> MKSNDMNITVELTFFEPYRLVEWFDWDARKKSHSAMRGQAFAQWTWKGKGRTAGKSFITGTLVRSAVIKAVEELLSLNNGKWEGVPCCNGSFQTDESKGKKPSFLRKRHTLQWQANNKNICDKEEACPFCILLGRFDNAGKVHERNKDYDIHFSNFDLDHKQEKNDLRLVDIASGRILNRVDFDTGKAKDYFRTWEADYETYGTYTGRITLRNEHAKKLLLASLGFVDKLCGALCRIEVIKKSESPLPSDTKEQSYTKDDTVEVLSEDHNDELRKQAEVIVEAFKQNDKLEKIRILADAIRTLRLHGEGVIEKDELPDGKEERDKGHHLWDIKVQGTALRTKLKELWQSNKDIGWRKFTEMLGSNLYLIYKKETGGVSTRFRILGDTEYYSKAHDSEGSDLFIPVTPPEGIETKEWIIVGRLKAATPFYFGVQQPSDSIPGKEKKSEDSLVINEHTSFNILLDKENRYRIPRSALRGALRRDLRTAFGSGCNVSLGGQILCNCKVCIEMRRITLKDSVSDFSEPPEIRYRIAKNPGTATVEDGSLFDIEVGPEGLTFPFVLRYRGHKFPEQLSSVIRYWEENDGKNGMAWLGGLDSTGKGRFALKDIKIFEWDLNQKINEYIKERGMRGKEKELLEMGESSLPDGLIPYKFFEERECLFPYKENLKPQWSEVQYTIEVGSPLLTADTISALTEPGNRDAIAYKKRVYNDGNNAIEPEPRFAVKSETHRGIFRTAVGRRTGDLGKEDHEDCTCDMCIIFGNEHESSKIRFEDLELINGNEFEKLEKHIDHVAIDRFTGGALDKAKFDTYPLAGSPKKPLKLKGRFWIKKGFSGDHKLLITTALSDIRDGLYPLGSKGGVGYGWVAGISIDDNVPDDFKEMINKTEMPLPEEVEESNNGPINNDYVHPGHQSPKQDHKNKNIYYPHYFLDSGSKVYREKDIITHEEFTEELLSGKINCKLETLTPLIIPDTSDENGLKLQGNKPGHKNYKFFNINGELMIPGSELRGMLRTHFEALTKSCFAIFGEDSTLSWRMNADEKDYKIDSNSIRKMESQRNPKYRIPDELQKELRNSGNGLFNRLYTSERRFWSDVSNKFENSIDYKREILRCAGRPKNYKGGIIRQRKDSLMAEELKVHRLPLYDNFDIPDSAYKANDHCRKSATCSTSRGCRERFTCGIKVR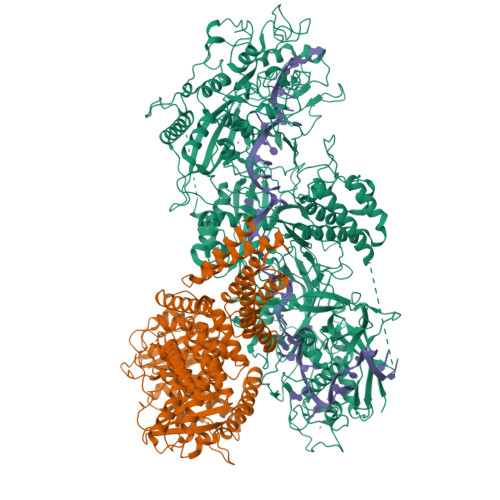DKNRVFLNAANNNRQYLNNIKKSNHDLYLQYLKGEKKIRFNSKVITGSERSPIDVIAELNERGRQTGFIKLSGLNNSNKSQGNTGTTFNSGWDRFELNILLDDLETRPSKSDYPRPRLLFTKDQYEYNITKRCERVFEIDKGNKTGYPVDDQIKKNYEDILDSYDGIKDQEVAERFDTFTRGSKLKVGDLVYFHIDGDNKIDSLIPVRISRKCASKTLGGKLDKALHPCTGLSDGLCPGCHLFGTTDYKGRVKFGFAKYENGPEWLITRGNNPERSLTLGVLESPRPAFSIPDDESEIPGRKFYLHHNGWRIIRQKQLEIRETVQPERNVTTEVMDKGNVFSFDVRFENLREWELGLLLQSLDPGKNIAHKLGKGKPYGFGSVKIKIDSLHTFKINSNNDKIKRVPQSDIREYINKGYQKLIEWSGNNSIQKGNVLPQWHVIPHIDKLYKLLWVPFLNDSKLEPDVRYPVLNEESKGYIEGSDYTYKKLGDKDNLPYKTRVKGLTTPWSPWNPFQVIAEHEEQEVNVTGSRPSVTDKIERDGKMV;> MNNTEENIDRIQEPTREDIDRKEAERLLDEAFNPRTKPVDRKKIINSALKILIGLYKEKKDDLTSASFISIARAYYLVSITILPKGTTIPEKKKEALRKGIEFIDRAINKFNGSILDSQRAFRIKSVLSIEFNRIDREKCDNIKLKNLLNEAVDKGCTDFDTYEWDIQIAIRLCELGVDMEGHFDNLIKSNKANDLQKAKAYYFIKKDDHKAKEHMDKCTASLKYTPCSHRLWDETVGFIERLKGDSSTLWRDFAIKTYRSCRVQEKETGTLRLRWYWSRHRVLYDMAFLAVKEQADDEEPDVNVKQAKIKKLAEISDSLKSRFSLRLSDMEKMPKSDDESNHEFKKFLDKCVTAYQDGYVINRSEDKEGQGENKSTTSKQPEPRPQAKLLELTQVPEGWVVVHFYLNKLEGMGNAIVFDKCANSWQYKEFQYKELFEVFLTWQANYNLYKENAAEHLVTLCKKIGETMPFLFCDNFIPNGKDVLFVPHDFLHRLPLHGSIENKTNGKLFLENHSCCYLPAWSFASEKEASTSDEYVLLKNFDQGHFETLQNNQIWGTQSVKDGASSDDLENIRNNPRLLTILCHGEANMSNPFRSMLKLANGGITYLEILNSVKGLKGSQVILGACETDLVPPLSDVMDEHYSVATALLLIGAAGVVGTMWKVRSNKTKSLIEWKLENIEYKLNEWQKETGGAAYKDHPPTFYRSIAFRSIGFPL>MGVTKTPLYETLNESSAVALAVKLGLFPSKSTLTCQEIGDGNLNYVFHIYDQEHDRALIIKQAVPYAKVVGESWPLTIDRARIESSALIRQGEHVPHLVPRVFYSDTEMAVTVMEDLSHLKIARKGLIEGENYPHLSQHIGEFLGKTLFYSSDYALEPKVKKQLVKQFTNPELCDITERLVFTDPFFDHDTNDFEEELRPFVEKLWNNDSVKIEAAKLKKSFLTSAETLIHGDLHTGSIFASEHETKVIDPEFAFYGPIGFDVGQFIANLFLNALSRDGADREPLYEHVNQVWETFEETFSEAWQK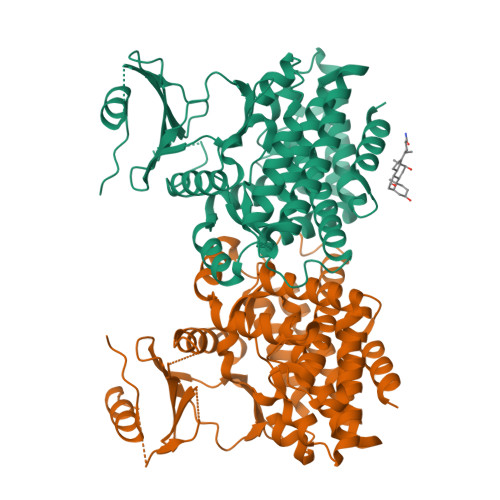DSLDVYANIDGYLTDTLSHIFEEAIGFAGCELIRRTIGLAHVADLDTIVPFDKRIGRKRLALETGTAFIEKRSEFKTITDVIELFKLLVKE[2x]> GPGSEFCADQYWNEVAVIDAIPLAATEHDTMLEMSDMQVWSAGDHPPIVSEEDISGSLVPRGSGSKSDSNASFLRAARAGNLDKVVEYLKGGIDINTCNQNGLNALHLAAKEGHVGLVQELLGRGSSVDSATKKGNTALHIASLAGQAEVVKVLVKEGANINAQSQNGFTPLYMAAQENHIDVVKYLLENGANQSTATEDGFTPLAVALQQGHNQAVAILLENDTKGKVRLPALHIAARKDDTKSAALLLQNDHNADVQSKMMVNRTTESGFTPLHIAAHYGNVNVATLLLNRGAAVDFTARNGITPLHVASKRGNTNMVKLLLDRGGQIDAKTRDGLTPLHCAARSGHDQVVELLLERGAPLLARTKNGLSPLHMAAQGDHVECVKHLLQHKAPVDDVTLDYLTALHVAAHCGHYRVTKLLLDKRANPNARALNGFTPLHIACKKNRIKVMELLVKYGASIQAITESGLTPIHVAAFMGHLNIVLLLLQNGASPDVTNIRGETALHMAARAGQVEVVRCLLRNGALVDARAREEQTPLHIASRLGKTEIVQLLLQHMAHPDAATTNGYTPLHISAREGQVDVASVLLEAGAAHSLATKKGFTPLHVAAKYGSLDVAKLLLQRRA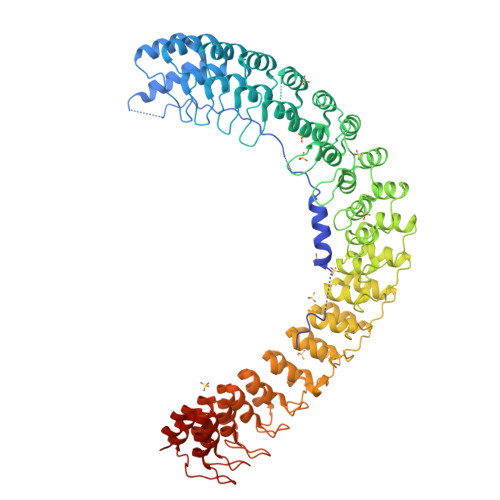AADSAGKNGLTPLHVAAHYDNQKVALLLLEKGASPHATAKNGYTPLHIAAKKNQMQIASTLLNYGAETNIVTKQGVTPLHLASQEGHTDMVTLLLDKGANIHMSTK Mitochondrial fission is a critical cellular event to maintain organelle function. This multistep process is initiated by the enhanced recruitment and oligomerization of dynamin-related protein 1 (Drp1) at the surface of mitochondria. As a member of the dynamin superfamily of proteins (DSPs), controlled Drp1 self-assembly into large helical polymers stimulates its GTPase activity to promote membrane constriction. All DSPs have two common domains, a GTPase or G domain, where GTP binding and hydrolysis occurs, and the stalk, comprised of the middle domain and GTPase effector domain (GED), which together drive self-assembly. Dynamin-related protein 1 (Drp1), the master regulator of mitochondrial fission, has a unique intervening sequence adjacent to the stalk called the variable domain (VD), composed of 136 intrinsically disordered residues that confer lipid sensing.

Here we present a cryo-EM structure of a full-length Drp1 dimer in an auto-inhibited state. Using cryo-EM, the structure of a full-length dimer of WT human Drp1 was resolved to a reported resolution of 5.97 Å and a 3DFSC resolution of 6.07 Å, which prevents the identification of side chains but secondary structure can be observed in regions of the map. Conformation 1 generated the highest quality map with the most particles, the best fit, and is used as the model dimer after applying a low pass filter of 6 Å to remove over-fitting artifacts. Overall, the architecture of the model dimer presents a compact organization of the GTPase and stalk domains, resulting in a ~ 100 Å decrease in length of the solution dimer when compared to the length of the crystal structure dimer with the VD deletion and GPRP401-404AAAA mutation. Specifically, hinge 1, comprised of two disordered loops that connect the BSE to the distal end of the stalk, adopts a conformation that places the GTPase domain near its own stalk. Comparing the autoinhibited dimer structure to the published crystal structure, the G domain of the cryo-EM structure is positioned 79 Å closer to the distal end of the stalk. The residues that form the discrete dimer interface identified by the Daumke group remain at the core of this dimer conformation;9 however, the density reveals additional burial of surface area between adjacent stalks in this region. In the solution (i.e., “closed”) state, L2S is juxtaposed to α1Ns, and this interaction requires a conformation with an obtuse angle between adjacent stalks (ranging from 103 to 145°) to form a more continuous interface. Helices α1CS and α1NS and loops L1NS and L2S would prevent the dimeric cryoEM structure from forming either interface without undergoing conformational rearrangements.

>MEALIPVINKLQDVFNTVGADIIQLPQIVVVGTQSSGKSSVLESLVGRDLLPRGTGIVTRRPLILQLVHVSQEDKRKTTGEENGVEAEEWGKFLHTKNKLYTDFDEIRQEIENETERISGNNKGVSPEPIHLKIFSPNVVNLTLVDLPGMTKVPVGDQPKDIELQIRELILRFISNPNSIILAVTAANTDMATSEALKISREVDPDGRRTLAVITKLDLMDAGTDAMDVLMGRVIPVKLGIIGVVNRSQLDINNKKSVTDSIRDEYAFLQKKYPSLANRNGTKYLARTLNRLLMHHIRDCLPELKTRINVLAAQYQSLLNSYGEPVDDKSATLLQLITKFATEYCNTIEGTAKYIETSELCGGARICYIFHETFGRTLESVDPLGGLNTIDILTAIRNATGPRPALFVPEVSFELLVKRQIKRLEEPSLRCVELVHEEMQRIIQHCSNYSTQELLRFPKLHDAIVEVVTCLLRKRLPVTNEMVHNLVAIELAYINTKHPDFADACGLMNNNIEEQRRNRLARELPSAVSRDKSSKVPSALAPASQEPSPAASAEADGKLIQDSRRETKNVASGGGGVGDGVQEPTTGNWRGMLKTSKAEELLAEEKSKPIPIMPASPQKGHAVNLLDVPVPVARKLSAREQRDCEVIERLIKSYFLIVRKNIQDSVPKAVMHFLVNHVKDTLQSELVGQLYKSSLLDDLLTESEDMAQRRKEAADMLKALQGASQIIAEIRETHLW[2x]> MSSLQKRPGPGNSSQPTERPRKESILDLS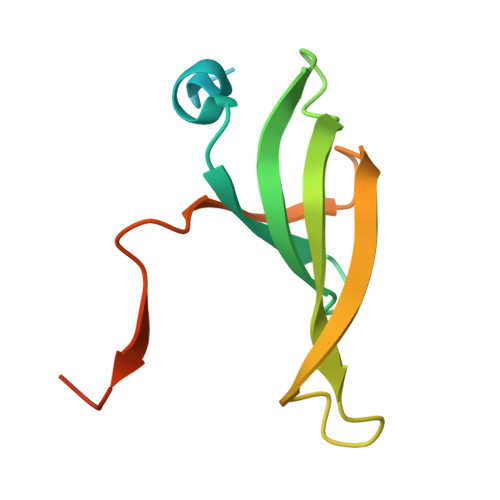RYQDQRIQATFTGGRQITGILKGFDQLMNLVLDDVEEQLRNPEDGKLTGAIRKLGLVVVRGTTLVLIAPMDGSEEIPNPFVQAEHHHHHH> MRGS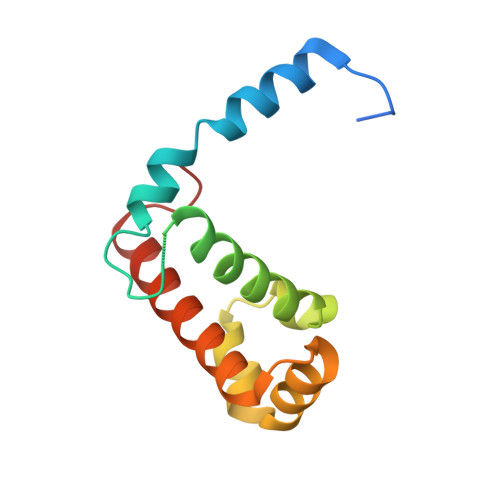HHHHHHKHGQFTLRDMYEQFQNIMKMGPFSQILGMIPGFGTDFMSKGNEQESMARLKKLMTIMDSMNDQELDSTDGAKVFSKQPGRIQRVARGSGVSTRDVQELLTQYTKFAQMVKKMGGIKGLF> GIREVILCKDQDGKIGLRLKSVDNGIFVQLVQANSPASLVGLRFGDQVLQINGE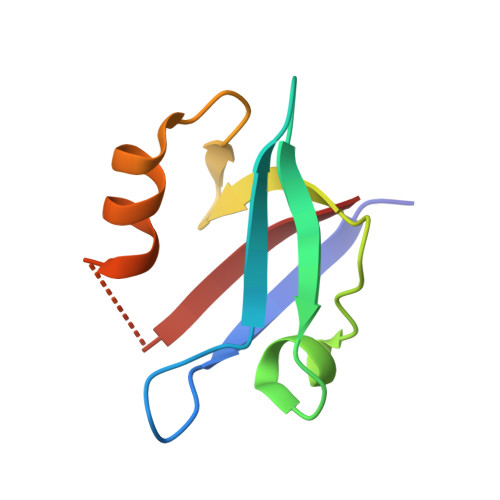NCAGWSSDKAHKVLKQAFGEKITMTIR>[5x]MQIYEGKLTAEGLRFGIVASRFNHALVDRLVEGAIDCIVRHGGREEDITLVRVPGSW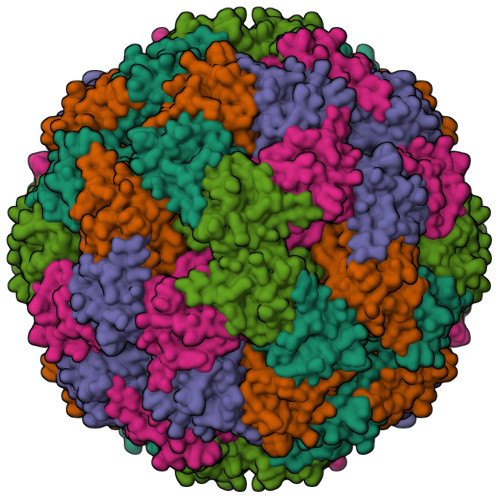EIPVAAGELARKEDIDAVIAIGVLIRGATPHFDYIASEVSKGLANLSLELRKPITFGVITADTLEQAIERAGTKHGNKGWEAALSAIEMANLFKSLR>[4x]MNPESRVIRKVLALQNDEKIFSGERRVLIAFSGGVDSVVLTDVLLKLKNYFSLKEVALAHFNHMLRESAERDEEFCKEFAKERNMKIFVGKEDVRAFAKENRMSLEEAGRFLRYKFLKEILESEGFDCIATAHHLNDLLETS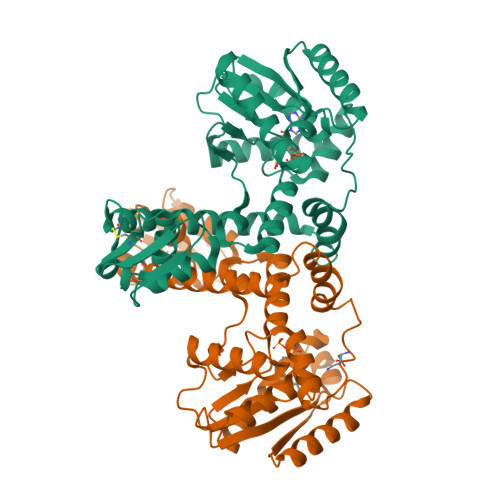LLFFTRGTGLDGLIGFLPKEEVIRRPLYYVKRSEIEEYAKFKGLRWVEDETNYEVSIPRNRIRHRVIPELKRINENLEDTFLKMVKVLRAEREFLEEEAQKLYKEVKKGNCLDVKKLKEKPLALQRRVIRKFIGEKDYEKVELVRSLLEKGGEVNLGKGKVLKRKERWLCFSPEV>MVSEPKVPKAPRPPKQPNVQDFQFFPPRLFELLEKEILYYRKTIGYKVPRNPDLPNSAQVQKEEQLKIDEAEPLNDEELEEKEKLLTQGFTNWNKRDFNQFIKANEKWGRDDIENIAREVEGKTPEEVIEYSAVFWERCNELQDIEKTMA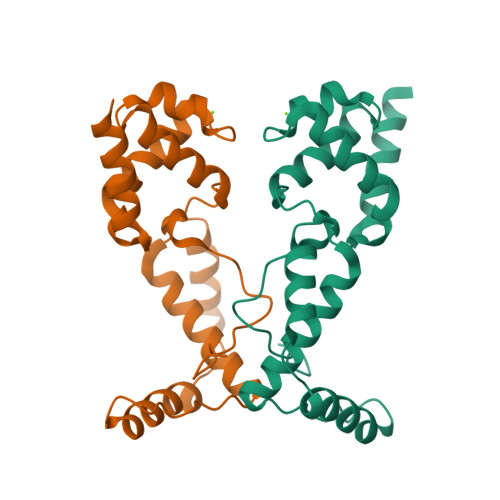QIERGEARIQRRISILEHHHHHH[2x]>MKTEQQIADIVNRTITPLMQEQAIPGMAVAVIYQGKPYYFTWGKADIANNHPVTQQTLFELGSVSKTFNGVLGGDAIARGEIKLSDPVTKYWPELTGKQWQGIRLLHLATYTEGGLPLKIPDDVRDKAALLHFYQNWQPQWTPGAKRLYANSSIGLFGALAVKPSGMSYEEAMTRRVLQPLKLAHTWITVPQNEQKDYAWGYREGKPVHSSPGQLDAEAYGVKSSVIDMARWVQANMDASHVQEKTLQQGIALAQSRYWRIGDMYQGLGWEMLNWPLKADSIINGSDSKVALAALPAVEVNPPAPAVKASWVHKTGSTGGFGSYVAFVPEKNLGIVMLANKSYPYPVRVEAAWRILEKLQ[2x]

CMY-185 is a CMY-2-like β-lactamase and was identified in an Escherichia coli clinical strain isolated from a patient who underwent treatment with ceftazidime-avibactam. CMY-185, possessing four amino acid substitutions of A114E, Q120K, V211S, and N346Y relative to CMY-2, confers high-level ceftazidime-avibactam resistance, and accumulation of the substitutions incrementally enhances the level of resistance to this agent. The substituted Y346 residue is a major driver of the functional evolution as it rejects primary avibactam binding due to the steric hindrance and augments oxyimino-cephalosporin hydrolysis through a drastic structural change, rotating the side chain of Y346 and then disrupting the H-10 helix structure. The other substituted residues E114 and K120 incrementally contribute to rejection of avibactam inhibition, while S211 stimulates the turnover rate of the oxyimino-cephalosporin hydrolysis.

We prepared the crystals of the CMY-185-ceftazidime complex by soaking a crystal of the CMY-185 free-form in mother liquor containing 100 mM ceftazidime for 4 h. Crystal structure of the CMY-185-ceftazidime complex showed an acyl-enzyme intermediate where the S64 catalytic residue is covalently bound to the C8 atom of ceftazidime, and its β-lactam structure is cleaved. In contrast to the free form, crystal structure of the CMY-185-ceftazidime complex revealed a drastic structural change of the R2 loop in that the H-10 helix was disrupted and disordered at residues N285–L293. In comparing the crystal structures of the CMY-185 free form and its complex, the C4 carboxyl group on the dihydrothiazine ring of ceftazidime occupied the position of the side chain of Y346 observed in the free form. The side chain of Y346 in the complex in turn was rotated 108° toward the H-10 helix and positioned to clash with the S287 residue, and this appeared to cause the disruption of the H-10 helix structure. We did not observe overall structural changes except for the R2 loop with the RMSD value of 0.68 Å, and the positions of the substituted residues E114, K120, and S211 were almost identical. The residues I284–L293 almost correspond to the disordered residues in the crystal structure of the CMY-185-ceftazidime complex, suggesting that, in the crystal, the fragile structure was entirely disrupted by the complex formation, without the influence of crystal packing. Our structural studies presented here clearly demonstrate that the ceftazidime molecule is bound to CMY-185, and that this in turn leads to the drastic structural change of CMY-185 to accommodate the ceftazidime binding. The structural change of the R2 loop in CMY-185 leads to further expansion of the substrate binding site for cephalosporins, and this expansion is a major cause for the reduced susceptibility to cefiderocol of the strain. In the CMY-185-ceftazidime complex, the K120 residue formed a stable salt bridge with the D123 residue.>[6x]MLRRKPTRLELKLDDIE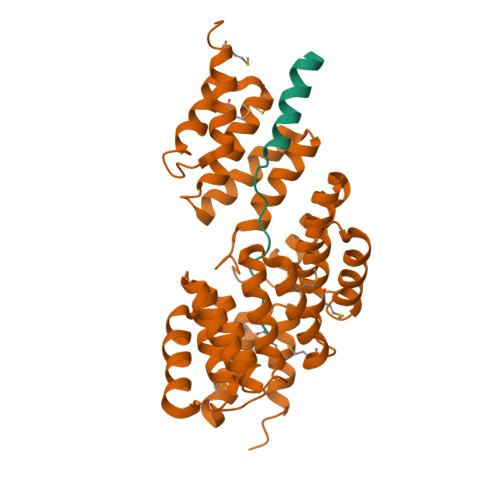EFENIRKDLETR;>GSYNKPSETVIPESVDGLQENLDVVVSLAERHYYNCDFKMCYKLTSVVMEKDPFHASCLPVHIGTLVELNKANELFYLSHKLVDLYPSNPVSWFAVGCYYLMVGHKNEHARRYLSKATTLEKTYGPAWIAYGHSFAVESEHDQAMAAYFTAAQLMKGCHLPMLYIGLEYGLTNNSKLAERFFSQALSIAPEDPFVMHEVGVVAFQNGEWKTAEKWFLDALEKIKAIGNEVTVDKWEPLLNNLGHVCRKLKKYAEALDYHRQALVLIPQNASTYSAIGYIHSLMGNFENAVDYFHTALGLRRDDTFSVTMLGHCIEMYIGDSEAYIGADIK[6x]> MRIERVDDTTVKLFITYSDIEARGFSREDLWTNRKRGEEFFWSMMDEINEEEDFVVEGPLW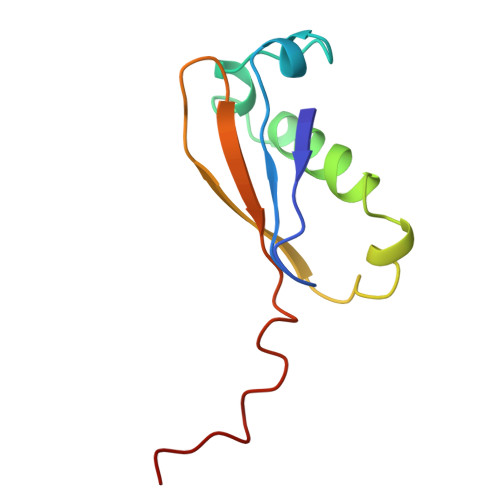IQVHAFEKGVEVTISKSKNEDMMNMSDDD6-{[3-(3-aminopropoxy)phenoxy]methyl}-4-methylpyridin-2-amine 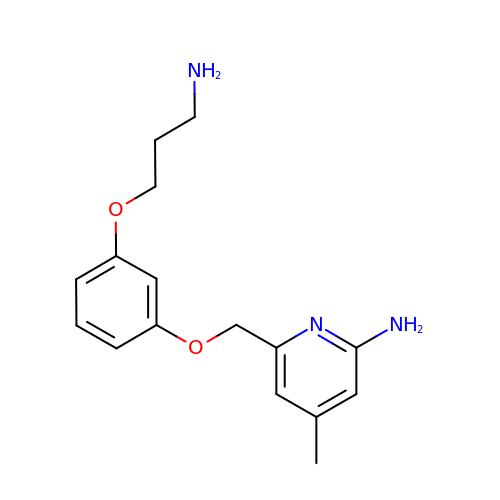| C16 H21 N3 O2 | USONDHXIUNXLQT-UHFFFAOYSA-N> MKQFGLAAFDELKDGKYNDVNKTILEKQSVELRDQLMVFQERLVEFAKKHNSELQASPEFRSKFMHMCSSIGIDPLSLFDRDKHLFTVNDFYYEVCLKVIEICRQTKDMNGGVISFQELEKVHFRKLNVGLDDLEKSIDMLKSLECFEIFQIRGKKFLRSVPNELTSDQTKILEICSILGYSSISLLKANLGWEAVRSKSALDEMVANGLLWIDYQGGAEALYWDPSWITRQL;>MSALPPVYSFPPLYTRQPNSLTRRQQISTWIDIISQYCKTKKIWYMSVDGTVINDNELDSGSTDNDDSKKISKNLFNNEDIQRSVSQVFIDEIWSQMTKEGKCLPIDQSGRRSSNTTTTRYFILWKSLDSWASLILQWFEDSGKLNQVITLYELSEGDETVNWEFHRMPESLLYYCLKPLCDRNRATMLKDENDKVIAIKVV[2x];> MEYWHYVETTSSGQPLLREGEKDIFIDQSVGLYHGKSKILQRQRGRIFLTSQRIIYIDDAKPTQNSLGLELDDLAYVNYSSGFLTRSPRLILFFKDPSSKDELGKSAETASADVVSTWVCPICMVSNETQGEFTKDTLPTPICINCGVPADYELT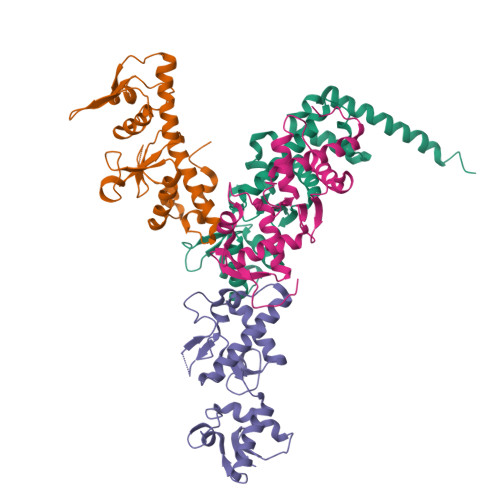KSSINCSNAIDPNANPQNQFGVNSENICPACTFANHPQIGNCEICGHRLPNASKVRSKLNRLNFHDSRVHIELEKNSLARNKSSHSALSSSSSTGSSTEFVQLSFRKSDGVLFSQATERALENILTEKNKHIFNQNVVSVNGVDMRKGASSHEYNNEVPFIETKLSRIGISSLEKSRENQLLNNDILFNNALTDLNKLMSLATSIERLYKNSNITMKTKTLNLQDESTVNEPKTRRPLLILDREKFLNKELFLDEIAREIYEFTLSEFKDLNSDTNYMIITLVDLYAMYNKSMRIGTGLISPMEMREACERFEHLGLNELKLVKVNKRILCVTSEKFDVVKEKLVDLIGDNPGSDLLRLTQILSSNNSKSNWTLGILMEVLQNCVDEGDLLIDKQLSGIYYYKNSYWPSHI>[2x]SMAEINEVVVVGMARTPIGRYLGGLASVRANDLAIIAANAAIERAGVDPGIIDEIVGATCLHAGNGSLP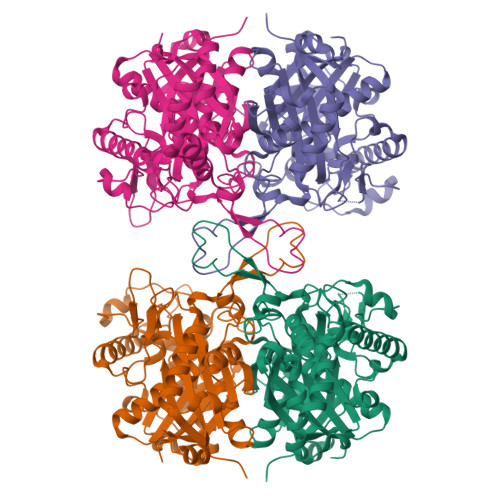PRIIGMKVGLPVRSGSCMVSQNCASGMRATEIACQNIMLGKTDISLVTAVESMSNIPYLLQQARSGYRMGDGKVQDAMLSDGLVCQLAGGHMGMTAENIAEKYGITREECDALALTSHQNAVKAVDEGIFDREIVPVVIKSKKGDKVISKDEHPIRGASLETMAKLPPAFKKGGVVTAANASGINDCAAAAVFMSKKKCEELGLKPLMKLVGICSEGVDAKVMGLGPAVAMPKVLKQAGWKYEDVDYWEVNEAFAAQVLGVVRMLKEEAGIELDFSKTNHNGSGIGLGHPVGATGLRIIVSMYYELERLGLTKGGASLCVGGGSAMASLWTRDI>TGAAPADAGSGLPALYREAVRTGRAAEMAE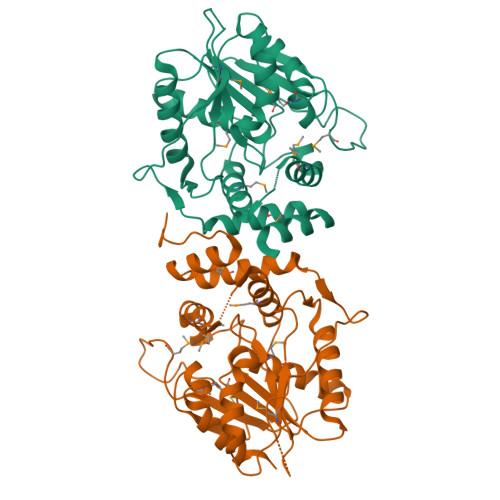LLAAASRFRPAFGTADRQPVALVPLADGAEDTGLPLLVGCAGTAVASGPVEFTAFAGALADLPAAAPMAALPQPGFLPGERVPATPEALFEAQAEALLRYAAGRPFVLLGHSAGANMAHALTRHLEANGGGPAGLVLMDIYTPADPGAMGVWRNDMFQWVWRRSDIPPDDHRLTAMGAYHRLLLDWSPTPVRAPVLHLRAAEPMGDWPPGDTGWQSHWDGAHTTAGIPGNHFTMMTEHASAAARLVHGWLA[2x]> AFLDNPTIILAHIRQSHVTSDDTGMCEMVLIDHDVDLEKIHPPSMPGDSGSEIQGSNGETQGYVYAQSVDITSSWDFGIRRRSNTAQRLERLRKERQNQIKCKNIQWKERNSKQSAQELKSLFEKKSLKEKPPISGKQSILSVRLEQCPLQLNNPFNEYSKFDGKGHVGTTATKKIDVYLPLHSSQDRLLPMTVVTMASARVQDLIGLICWQYTSEGREPKLNDNVSAY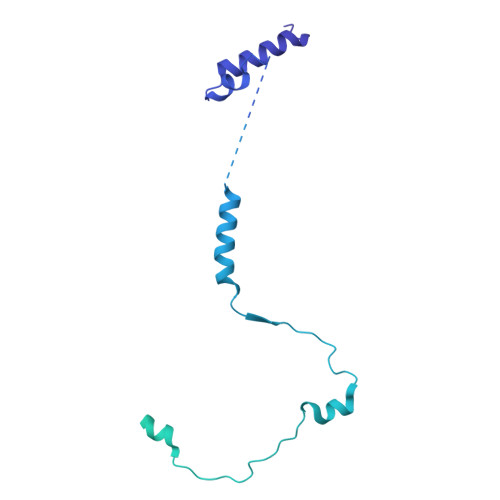CLHIAEDDGEVDTDFPPLDSNEPIHKFGFSTLALVEKYSSPGLTSKESLFVRINAAHGFSLIQVDNTKVTMKEILLKAVKRRKGSQKVSGPQYRLEKQSEPNVAVDLDSTLESQSAWEFCLVRENSSRADGVFEEDSQIDIATVQDMLSSHHYKSFKVSMIHRLRFTTDVQLGISGDKVEIDPVTNQKASTKFWIKQKPISIDSDLLCACDLAEEKSPSHAIFKLTYLSNHDYKHLYFESDAATVNEIVLKVNYILESRASTARADYFAQKQRKLNRRTSFSFQKEKKSGQQ>AMPLDAGGQNSTQMVLAPGASIFRCRQCGQTISRRDWLLPMGGDHEHVVFNPAGMIFRVWCFSLAQGLRLIGAPSGEFSWFKGYDWTIALCGQCGSHLG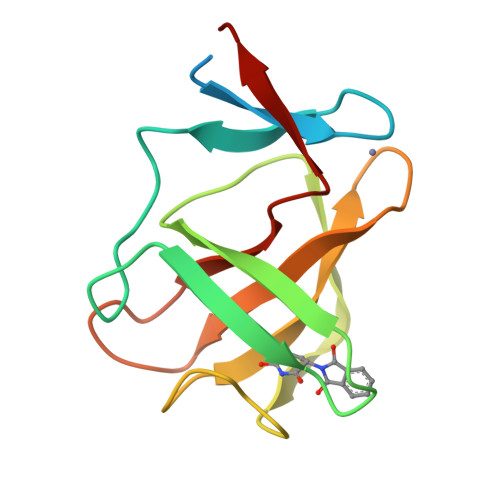WHFEGGSQPQTFFGLIKDRLAEGPAD[3x]2-azanyl-3-[[(2~{R})-oxolan-2-yl]methyl]-7-(5-phenylpentyl)quinazolin-4-one 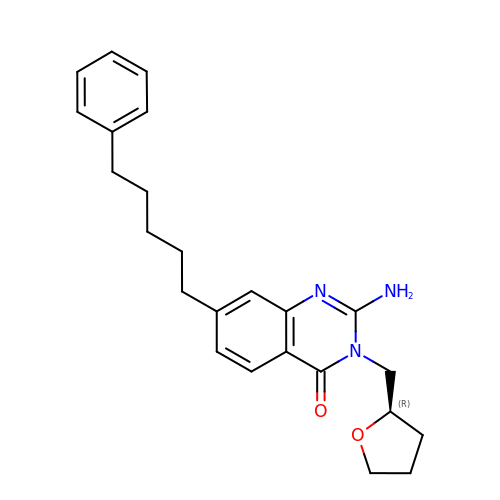| C24 H29 N3 O2 | RDQORSXQWHKSAX-HXUWFJFHSA-N1-[(3~{R})-3-[4-azanyl-3-[1-(2-phenylethyl)-1,2,3-triazol-4-yl]pyrazolo[3,4-d]pyrimidin-1-yl]piperidin-1-yl]propan-1-one 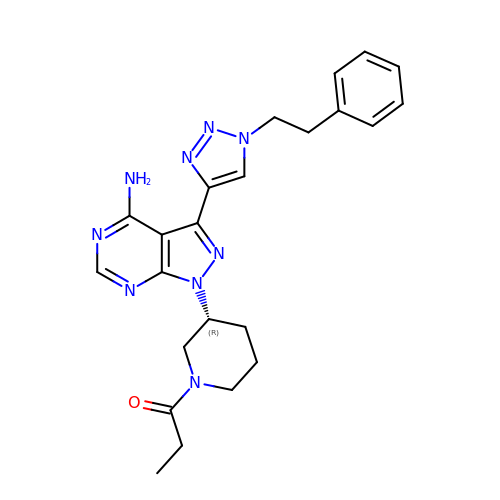| C23 H27 N9 O | DQBPZDXMZGPVRU-QGZVFWFLSA-N>[2x]GSMAFVKSGWLLRQSTILKRWKKNWFDLWSD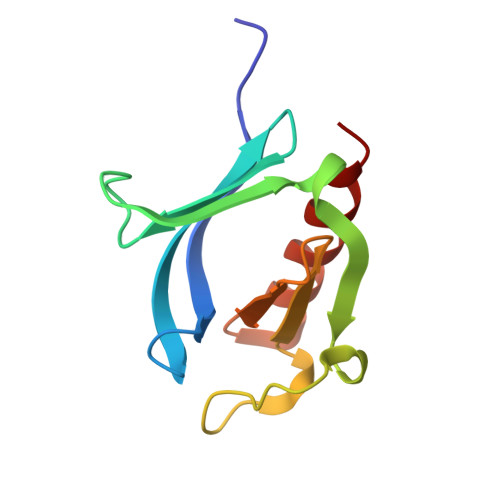GHLIYYDDQTRQNIEDKVHMPMDCINIRTGQECRDTQPPDGKSKDCMLQIVCRDGKTISLCAESTDDCLAWKFTLQDSRTN>[3x]MHHHHHHMPLEPHFMPDF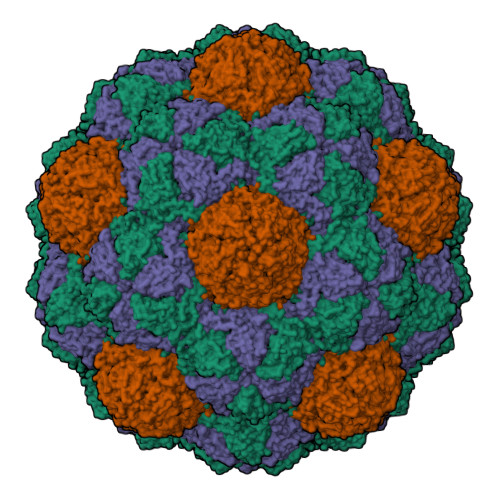LGHAENPLREEEWARLNETVIQVARRSLVGRRILDIYGPLGAGVQTVPYDEFQGVSPGAVDIVGEQETAMVFTDARKFKTIPIIYKDFLLHWRDIEAARTHNMPLDVSAAAGAAALCAQQEDELIFYGDARLGYEGLMTANGRLTVPLGDWTSPGGGFQAIVEATRKLNEQGHFGPYAVVLSPRLYSQLHRIYEKTGVLEIETIRQLASDGVYQSNRLRGESGVVVSTGRENMDLAVSMDMVAAYLGASRMNHPFRVLEALLLRIKHPDAICTLEGAGATERR;>[3x]GLTVGSLRG>[2x]GPLGSMAQSTVLPMHCLYGIFLEGNLKIQKNDQEGLKKFKDNIKKFTLELDEIDKISPQSRIGGAICFSSDIWDTVTKKISKPKELKSVNTLSSYMPGTSQRDILIHIISDRMDTCFKLAQDTMRNFGEDQLD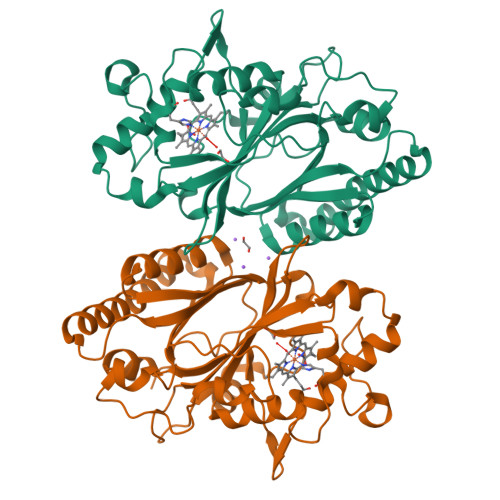IKQEIHGFRRVEERDLTDFIDGTENPDGDELRTQYGLVAAGQPNEFGSYVFTQRYVHNLKKWYPEPLSVQQDTVGRTKKDSIEIPRDKRPITSHVSRTDLSENGKDLKIVRQSLPYGQITGEKGLMFIAYACSLHNIEKQLQSMFGQLDGKHDLLLKYTTPVTGSFYFAPSKKELLEL> MHRVMGIETEYGISVPHQPNANAMAASSQVVNAYAPIGAPAQRQARWDFEEENPLRDARGFEVAREAADPSQLTDEDLGLANVILTNGARLYVDHAHPEYSTPEVTNPRDAVLWDKAGERIMAEAARRAADLPMGWTIQLYKNNTDNKGASYGCHENYLMNRSTPFADIVRHLIPFFVTRQVFCGAGRVGIGADGRGEGFQLSQRADFFEVEVGLETTLKRPIINTRDEPHADPEKYRRLHVIIGDANMSEIATYLKLGTTALVLAMIEDGFLSQDFSVESPVGALRAVSHDPTLRYQLRLHDGRRLTAVQLQMEYLEQARKYVEDRFGTDVDDMTRDVLDRWETTLVRLADDPMQLSRDLDWVAKLSILEGYRQRENLPWSAHKLQLVDLQYHDVRPDRGLYNRLVARGRMNLLVDEAAVRTAMHEPPNDTRAYFRGRCLAKFGAEIAAASWDSVIFDLPGRDSLQRVPTLEPLRGTRA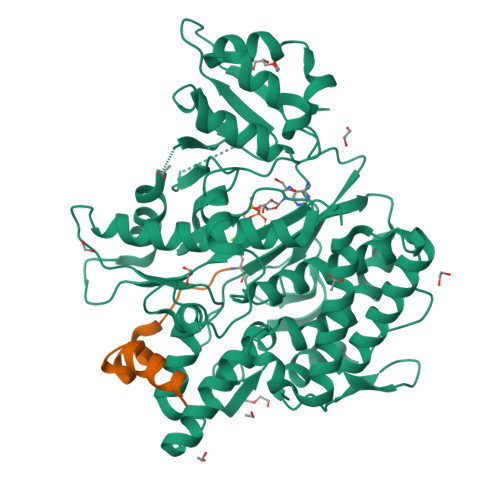HVGDLLDRCRSATELVAALTGGENLYFQ;> DAILDEIDDVLEENAEEFVRSYIQKGGE>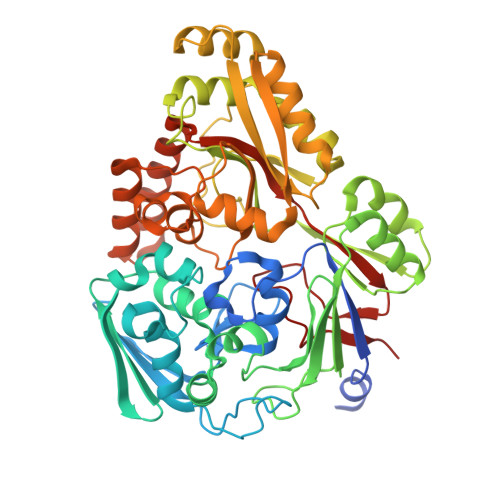 GIDPFTSENPNATLNPSKENISVKEQKRFGGVLVFARGADGSSMDPALVTDGESYVATGNIYDTLVQFKYGTTEIEPALATSWDISPDGLVYTFHLRKGVYFHQTKYWNKKVEFSAKDVLFSFERQMDKAKRYYSPGAKSYKYWEGMGMSHIIKSIEALDDYTIRFTLNGPEAPFLANLGMDFLSILSKDYADYLEQNNKKDELAKKPVGTGPFKFFLWNKDEKIILLKNQDYWGPKAYLDKVVVRTIPNSSTRALALRTGEIMLMTGPNLNEVEQLEKLPNIVVDKSAGLLASWLSLNTQKKYFNNPLVRLAINHAINVDDYIKVIYEGFAQKMVNPFPPTIWGYNYNIKPYEYDLKKAKELLKQAGYPNGFKTTIFTTSTRNPKGAVFIQASLAKIGIDVKIEVYEWGAYLKRTGLGEHEMAFAGWMADIADPDNFLYTLWSKQAASAIPTQNGSFYKSDAFSDLLIKAKRVSDQKEREALYLKAQEIIHKDAPYVPLAYPYSVVPHLSKVKGYKTTGVSVNRFFKVYLEK;> STSA> GNPLRKFKLVFLGEQSVGKTSLITRFMYDSFDNTYQATIGIDFLSKTMYLEDRTVRLQLWDTAGLERFRSLIPSYIRDSTVAVVVYDITNVNSFQQTTKWIDDVRTERGSDVIIMLVGNKTDLADKRQVSIEEGER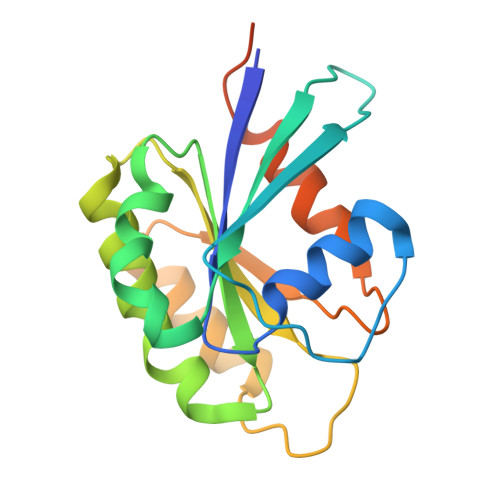KAKELNVMFIETSAKAGYNVKQLFRRVAAALPGMESTQDRSREDMIDIKLEK>MRILILGMGGTIASVKGERGYESALSVSKILKLAGISSEAKIEARDLMNVDSTLIQPSDWERLAKEIEKEVWEYDGIVITHGTDTMAYSASMLSFMLRNPPIPIVLTGSMLPITEKNSDAPFNLRTALEFVKLGIRGIYIAFNGKVMLGVRASKIRSMGFDAFESINYPNVAEIKDDKLRILHIPDFYGDEFFSDIKYEPKVLVIKLIPGLSGDIVREALRLGYKGIILEGYGVGGIPYRGTDLFEVVSSISKRIPVVLTTQAI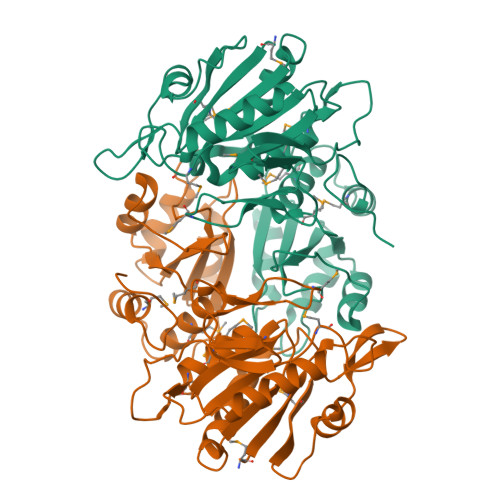YDGVDLQRYKVGRIALEAGVIPAGDMTKEATITKLMWILGHTKNIEEVKQLMGKNITGELTRVS[2x]>MKKHIIIKTIPKKEEIISRDLCDCIYYY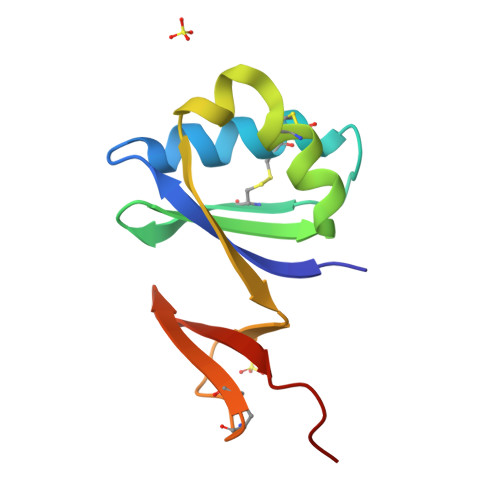DNSVICKPIGPSKVYVSTSLENLEKCLQLHYFKKLVKNIEIFDEVHNSKPNCDKCLIVEIGGVYFVRRVNGVPR[2x]>[4x]MKMEARQKQNSFTSKMQKIVNHRAFTFTVIALILFNALIVGIETYPRIYADHKWLFYRIDLVLLWIFTIE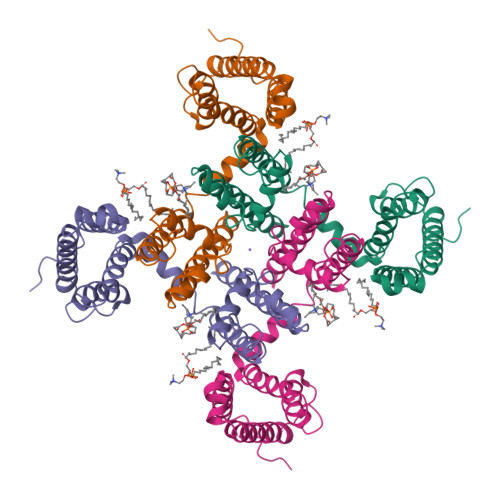IAMRFLASNPKSAFFRSSWNWFDFLIVAAGHIFAGAQFVTVLRILRVLRVLRAISVVPSLRRLVDALVMTIPALGNILILMSIFFYIFAVIGTMLFQHVSPEYFGNLQLSLLTLFQVVTLESWASGVMRPIFAEVPWSWLYFVSFVLIGTFIIFNLFIGVIVNNVEKAELTDNEEDGEADGLKQEISALRKDVAELKSLLKQSK>[3x]MVEVEHWNTLRLRIYIGENDKWEGRPLYKVIVEKLREMGIAG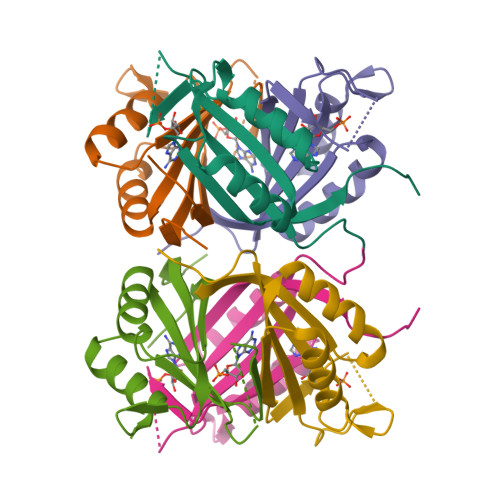ATVYRGIYGFGKKSRVHSSDVIRLSTDLPIIVEVVDRGHNIEKVVNVIKPMIKDGMITVEPTIVLWVGTQEEIKKFEEDAIAERQ>[2x]QTVEAMAQGLPAPSYW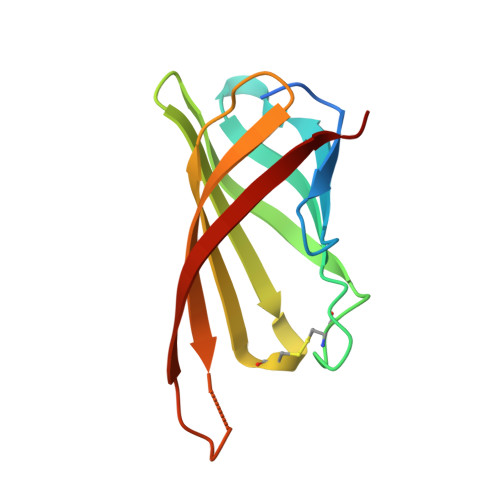KNERGSELLIWSANSGTIQGTFTNHAQGFACQGIPYPAAGSVSPTGLYFVVTFAQCNSFTRWVGTIKGSQMPTSWTLFYVDNKGKPSRLKGGDIFTRVW> NQPVNQPILAAAQSLHREATKWSSKGNDIIAAAKRMALLMAEMSRLVRGGSGTKRAL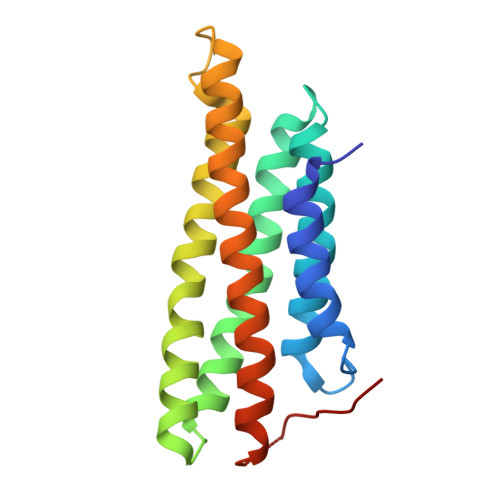IQCAKDIAKASDEVTRLAKEVAKQCTDKRIRTNLLQVCERIPTISTQLKILSTVKATMLGRTNISDEESEQATEMLVHNAQNLMQSVKETVREAEAASIKIRTDAGFTLRWVRKT N-cyclopropyl-N-(4-methyl-1,3-thiazol-2-yl)-2-[(6-phenylpyridazin-3-yl)sulfanyl]acetamide | C19 H18 N4 O S2 | 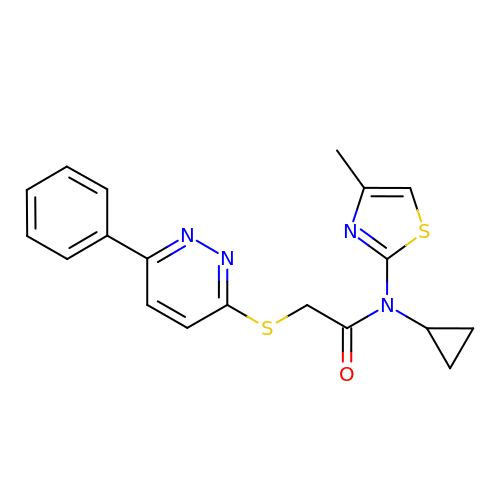DPONSKCACOZTGN-UHFFFAOYSA-N> SAKAVDYETEVVLGNGERKKIGEIVERAIEEAEKNGKLGRVDDGFYAPIDIEVYSLDLETLKVRKARANIAWKRTAPKKMMLVKTRGGKRIRVTPTHPFFVLEEGKVAMRKARDLEEGNKIATIEGLSVSWDEVAEILEYE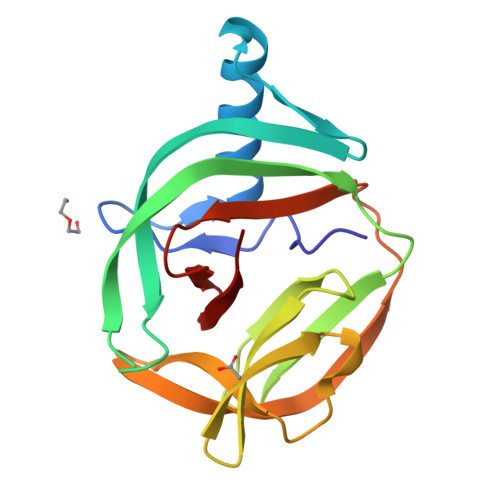PKDPWVYDLQVPGYHNFLANGIFVHAA(2S)-2-[[(2S)-2-(6-bromanyl-3-oxidanylidene-1H-isoindol-2-yl)-3-[4-(5-ethanoyl-2-fluoranyl-phenyl)phenyl]propanoyl]amino]propanoic 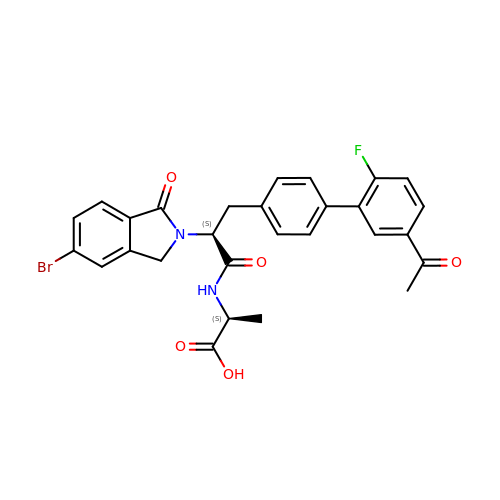acid | C28 H24 Br F N2 O5 | OIZONSTWGHXIOF-MQNRADLISA-N> GAMASGKVVKFSYMWTINNFSFCREKMGEVIKSSTFSSGANDKLKWCLRVNPKGLD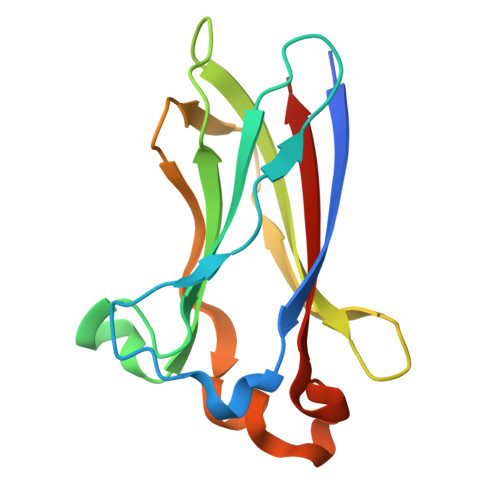EESKDYLSLYLLLVSCPKSEVRAKFKFSILNAKGEETKAMESQRAYRFVQGKDWGFKKFIRRDFLLDEANGLLPDDKLTLFCEVSVVQD>[10x]TPDCVTGKVEYTKYNDDDTFTVKVGD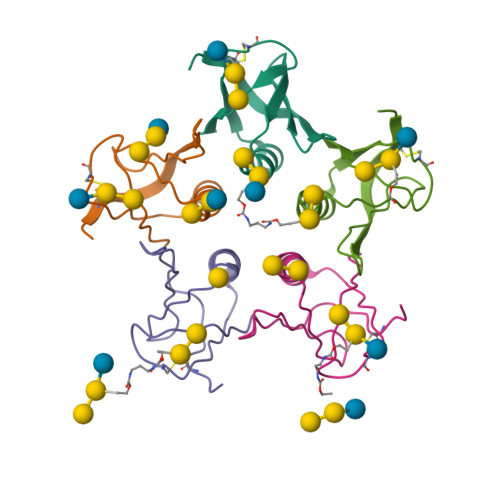KELFTNRWNLQSLLLSAQITGMTVTIKTNACHNGGGFSEVIFR Phosphopantetheine adenylyltransferase (PPAT) catalyzes the fourth of five steps in the coenzyme A biosynthetic pathway, reversibly transferring an adenylyl group from ATP onto 4′-phosphopantetheine to yield dephospho-coenzyme A and pyrophosphate. Dephospho-coenzyme A synthesis by PPAT is believed to be the rate-limiting step in CoA biosynthesis. In B. pseudomallei, the coaD gene encodes the 166-residue protein Bp PPAT, although it has not yet been shown that Bp PPAT is essential for B. pseudomallei. The crystal structure of Bp PPAT features a Rossmann fold, which is known to bind di­nucleotides as well as GTP and ATP.

From a protein sample concentrated in the presence of ATP, we solved a 2.1 Å resolution crystal structure of Bp PPAT. This structure had clear evidence but weak electron density for de­phospho-coenzyme A in the active site, indicating that dephospho-coenzyme A was only partially occupied. Coenzyme A metabolites are known to exist at significant concentrations in E. coli and thus it is not surprising to see dephospho-coenzyme A carried through the purification from the expression host. Refinement with the occupancy of dephospho-coenzyme A set to 0.5 (i.e. 50%) resulted in crystallographic B factors that were in line with those of the surrounding protein atoms (∼30 Å2). Dephospho-coenzyme A forms many packing interactions and hydrogen bonds with backbone amides in the active site, but also makes hydrogen bonds to the side chains of the conserved residues Thr9 (which is conserved as a threonine or serine), Arg87 (which is conserved as an arginine or lysine) and Glu98. One copy of Bp PPAT was observed in the asymmetric unit, indicating that the other five copies that comprise the biologically active homohexamer are crystallo­graphically equivalent. The overall structure and ligand-binding interactions are quite similar to other bacterial PPAT crystal structures.

> GPGSMVVAVYPGTFDPLTRGHEDLVRRASSIFDTLVVGVADSRAKKPFFSLEERLKIANEVLGHYPNVKVMGFTGLLKDFVRANDARVIVRGLRAVSDFEYEFQMAGMNRYLLPDVETMFMTPSDQYQFISGTIVREIAQLGGDVSKFVFPSVEKWLTEKVAAMAQGPSA>[2x]SNMDGRIVIVDDEPITRLDIRDIVIEAGYEVVGEAADGFEAIEVCKKTQPDLVLMDIQMPILDGLKAGKKIVQDQ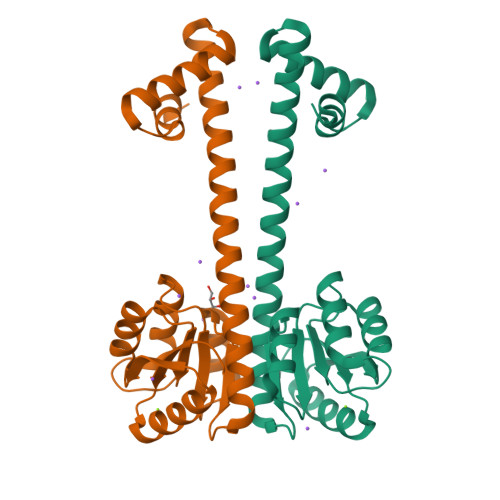LASSIVFLSAYSDVQNTDKAKKLGALGYLVKPLDEKSLIPTIEMSIERGKQTQLLLSQIDKLSLKLEERKIIEKAKGILVKENHISEEEAYQMLRTLSMNKRARMSEIAELIVMDDE>MDPPARKEKTKVKESVSRVEKAKQKSAQQELKQRQRAEIYALNRVMTELEQQQFDEFCKQMQPPGE[2x];>MDEATWERMWKHVAKIHPDGEKVAQRIRGATDLPKIPIPSVPTFQPSTPVPERLEAVQRYIRELQYNHTGTQFFEIKKSRPLTGLMDLAKEMTKEALPIKALEAVILGIYLTNSMPTLERFPISFKTYFSGNYFRHIVLGVNFAGRYGALGMSRREDLMYKPPAFRTLSELVLDFEAAYGRCWHVLKKVK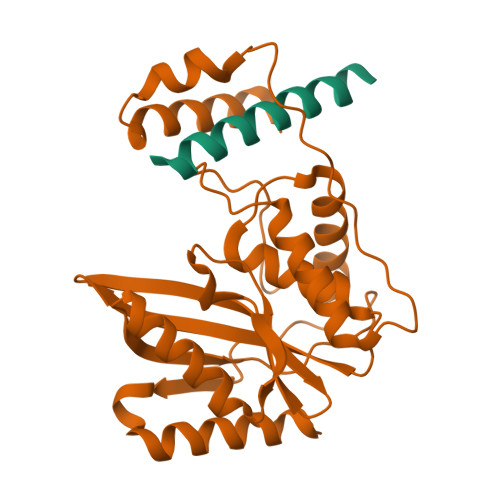LGQSVSHDPHSVEQIEWKHSVLDVERLGRDDFRKELERHARDMRLKIG[2x]>MNKDIATPIRTKEILKKYGFSFKKSLGQNFLIDTNILNRIVDHAEVTEKTGVIEIGPGIGALTEQLAKRAKKVVAFEIDQRLLPILKDTLSPYENVTVIHQDVLKADVKSVIEEQFQDC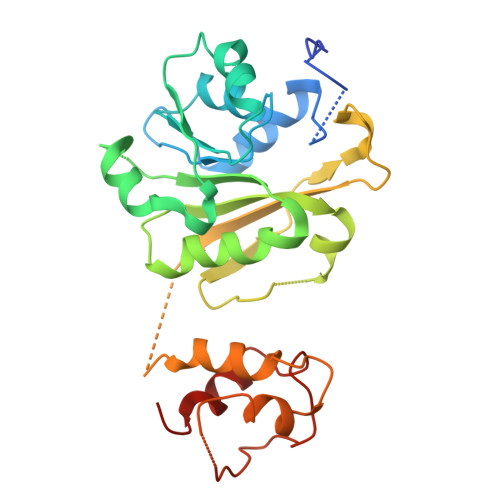DEIMVVANLPYYVTTPIIMKLLEEHLPLKGIVVMLQKEVAERMANTKRSLSIAVQFYTEAKTVMIVPKTVFVPQPNVDSAVIRLILRDGPAVDVENESFFFQLIKASFAQRRKTLLNNLVNNLPEGKAQKSTIEQVLEETNIDGKRRGESLSIEEFAALSNGLYKALF[2x]>MGHHHHHHGSPEDLSLEEREELLDIRRRKKELIDDIERLKYEIAEVMTEIDNLTSVEESKYTQRNAQIAMGRKKFNMDPKKGIQFLIENDLLQSSPEDVAQFLYKGEGLNKTVIGDYLGERDDFNIKVLQAFVELHEFADLNLVQALRQFLWSFRLPGEAQKIDRMMEAFASRYCLCNPGVFQSTDTCYVLSFAIIMLNTSLHNHNVRDKPTAERFITMNRGINEGGDLPEELLRNLYESIKNEPFKIPEDDGNDLTYTFFNPDREGWLLKLGGRVKTWKRRWFILTDNCLYYFEYTTDKEPR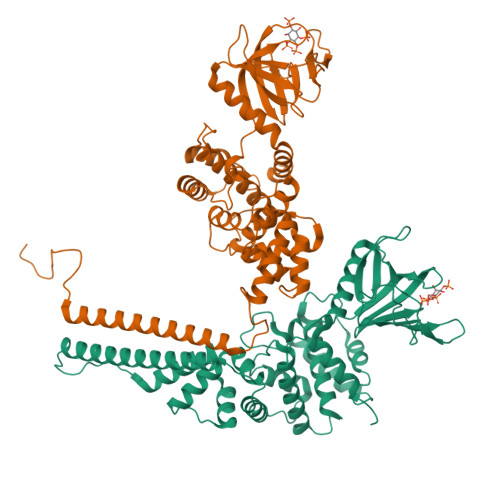GIIPLENLSIREVEDPRKPNCFELYNPSHKGQVIKACKTEADGRVVEGNHVVYRISAPSPEEKEEWMKSIKASISRDPFYDMLATRKRRIANKK[2x]>GSLKQESNDIGSGENNRARPCDTCRSNACTVYCHADSAYLCMSCDAQVHSANRVASRHKRVRVCESCERAPAAFLCEADDASLCTACDSEVHSANPLARRHQRVPILPISG[3x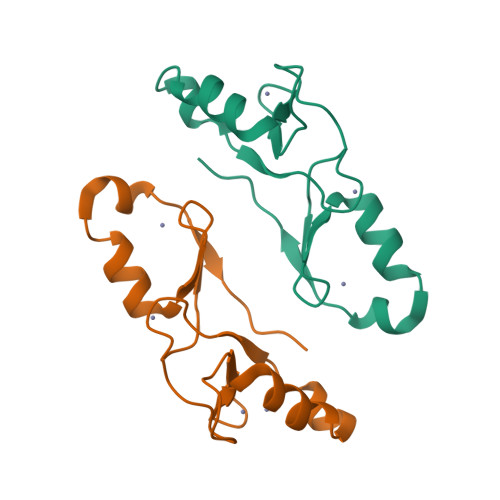]> MAGTDKRKQSLYFPEEMLKEIQEEATRQDRSLSWVVQQA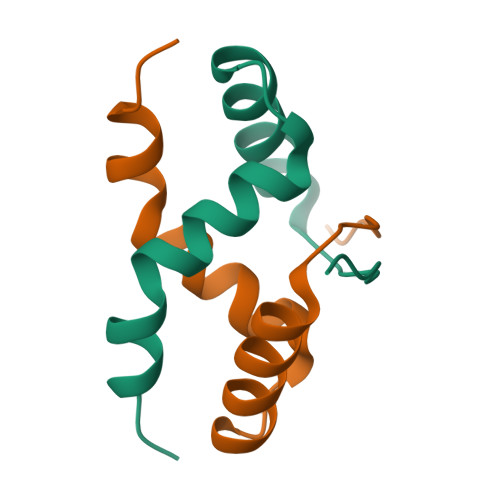WKIARERIKSFPAVNDVTGDERQDPREE> MGSDKIHHHHHHENLYFQGMHIHILGICGTFMGSLALLARALGHTVTGSDANIYPPMSTQLEQAGVTIEEGYLIAHLQPAPDLVVVGNAMKRGMDVIEYMLDTGLRYTSGPQFLSEQVLQSRHVIAVAGTHGKTTTTTMLAWILHYAGIDAGFLIGGVPLVNTTDTNLQQVFAHSSYLGTEKDDSDNSVNTGYFVIEADEYDSAFFDKRSKFVHYRPRTAILNNLEFDHADIFADLDAIQTQFHHMVRMIPSTGKIIMPAATISLEDTLAKGVWTPIWRTSVIDSTISSVRREDSPLENSQAENSSDWQAELISADGSQFTVSFNDNKEATALVNWSMSGLHNVNNALVAIAAAYNIGVSVKTACAALSAFAGIKRRMELIGDVNDILVFDDFAHHPTAITTTLDGAKKKLADRRLWAIIEPRSNTMKMGIHQDSLAQSATLADHTLWYEPTGLEWGLKEVIDNATIANPSIGSQQVLSSVDDIIKHICTHAKAGDAIVIMSNGGFEGIHQRLLTALGNIVAIL

Recycling of the bacterial cell wall is believed to account for ∼30–60% of peptidoglycan synthesis in Gram-negative bacteria. The Mpl protein is used to link the breakdown component, the tripeptide L-Ala-γ-D-Glu-meso-A2pm (and also tetra- and pentapeptides), to UDP-MurNAc. Mpl is functionally similar to MurC, as both mechanisms involve ligation of an amino acid or peptide to UDP-MurNAc; in MurC, a single amino acid (L-Ala) is attached and in Mpl, a tri-, tetra- or pentapeptide. Mpl and MurC-F enzymes have three domains that are classified in Pfam families, PF01225 (Mur ligase catalytic domain), PF08245 (Mur ligase middle domain) and PF02875 (Mur ligase glutamate binding/C-terminal domain).

In this study, we have determined the crystal structure of a full-length apo-Mpl protein from the permafrost bacterium Psychrobacter arcticus 273-4, PaMpl (UniProt accession code Q4FVQ2_PSYA2, locus name Psyc_0032, 505 amino acids) at 1.65 Å resolution and have also biochemically characterized this enzyme. The crystal structure of PaMpl was determined by Multi-wavelength Anomalous Diffraction (MAD) phasing to a resolution of 1.65 Å. PaMpl is present as a monomer in the crystal asymmetric unit. The final model includes Gly0 (a remnant from cleavage of the expression and purification tag); residues 1–209, 216–265, and 285–504 of the protein (the full-length protein contains 505 residues); and 588 water molecules. PaMpl can be divided into 3 distinct domains: the N-terminal UDP-MurNAc-binding domain (ND, residues 1–102), the middle ATP-binding domain (MD, residues 103–357) and the C-terminal tripeptide-binding domain (CD, residues 358–505). The CD is a six-stranded, mainly parallel β-sheet (β16–β21) flanked on one side by α-helices H14-H16 and 310-helix H17, and on the other by H18–H19. These 3 domains are linked contiguously to form a triangular-shaped molecule with dimensions of ∼56×60×47 Å3. The largest conformational difference is in the disposition of the CD in Mpl, which is rotated 30° relative to ND and MD, when compared to its disposition in MurC (respectively). The corresponding residue in PaMpl is His210, but this region (residues 210–215) is disordered in our structure, probably due to the absence of metal ions. A loop (residues 404–414) from CD in PaMpl is folded into part of the ATP and UDP-MurNAc binding site. Structure analyses indicate that the orientation of the CD domain of PaMpl relative to the other domains is flexible and changes on substrate binding.4-DIMETHYLAMINO-1,10,11,12-TETRAHYDROXY-3-OXO-3,4,4A,5-TETRAHYDRO-NAPHTHACENE-2-CARBOXYLIC 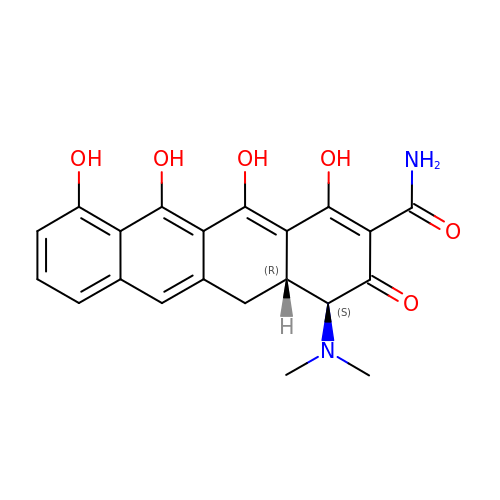ACID AMIDE | C21 H20 N2 O6 | CSMTWDGQMUIMDU-HWPZZCPQSA-N>GSHMNQCPEHSQLTTLGVDGKEFPEVHLGQWYFIAGAAPTKEELATFDPVDNIV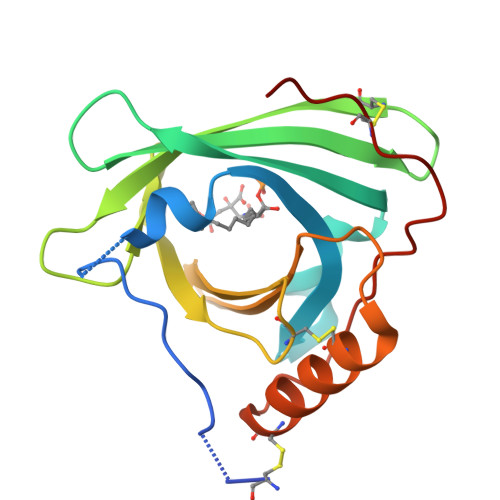FNMAAGSAPMQLHLRATIRMKDGLCVPRKWIYHLTEGSTDLRTEGRPDMKTELFSSSCPGGIMLNETGQGYQRFLLYNRSPHPPEKCVEEFKSLTSCLDSKAFLLTPRNQEACELSNN[2x]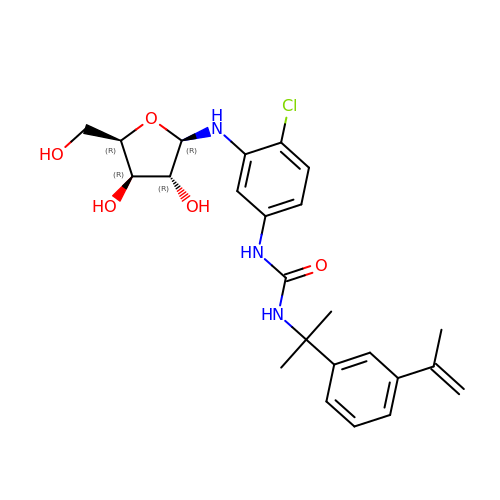N-{2-chloro-5-[({2-[3-(prop-1-en-2-yl)phenyl]propan-2-yl}carbamoyl)amino]phenyl}-beta-D-xylofuranosylamine | C24 H30 Cl N3 O5 | RGENKIJBZZZCQP-CIAFKFPVSA-N>APADNAADARPVDVSVSIFINKIYGVNTLEQTYKVDGYIVAQWTGKPRKTPGDKPLIVENTQIERWINNGLWVPALEFINVVGSPDTGNKRLMLFPDGRVIYNARFLGSFSNDMDFRLFPFDRQQFVLELEPFSYNNQQLRFSDIQVYTENIDNEEIDEWWIRGKASTHISDIRYDHLSSVQPNQNEFSRITVRIDAVRNPSYYLWSFILPLGLIIAASWSVFWLESFSERLQTSFTLMLTVVAYAFYTSNILGRLPYTTYIDQMIIAGYGSIFAAILLIIFAHHRQANGVEDDLLIQRSRLAFPLGFLAIGCVLVIRFFTL[5x]

Pentameric ligand-gated ion channels (pLGICs) mediate synaptic transmission and are sensitive to their lipid environment. We demonstrate that the model pLGIC, ELIC (Erwinia ligand-gated ion channel), is positively modulated by the anionic phospholipid, phosphatidylglycerol, from the outer leaflet of the membrane. To investigate the mechanism of positive modulation by POPG, we determined structures of WT ELIC by single particle cryo-electron microscopy (cryo-EM) in the absence and presence of agonist in MSP1E3D1 nanodiscs with 2:1:1 POPC:POPE:POPG (hereafter referred to as 2:1:1) or POPC. In combination with streamlined alchemical free energy perturbation calculations and functional measurements in asymmetric liposomes, the data support a mechanism by which an anionic phospholipid stabilizes the activated, open-channel state of a pLGIC by specific, state-dependent binding to this site.

Seeking a mutant that remains open in the presence of agonist, we added the mutations P254G (previously shown to slow deactivation) and C300S (previously shown to slow desensitization in the presence of agonist), and produced P254G/C300S/V261Y/G319F/I320F (ELIC5). Strikingly, ELIC5 showed a deactivation rate ~1000× slower than WT and no evidence of desensitization in the presence of 10 mM cysteamine, indicative of profound stabilization of the activated, open-channel state. Consistent with its gain-of-function phenotype, a structure of ELIC5 in 2:1:1 nanodiscs with 10 mM cysteamine, determined at 3.4 Å resolution, yielded an apparent open pore with a pronounced outer leaflet phospholipid-shaped density. Finally, in ELIC5, 9′ rotates away from the pore into an intersubunit space and 16′ opens further, such that the narrowest diameter of the pore is at 2′ (Q233). Two rotameric states of Q233 could be modeled in the structure yielding a minimum pore diameter of 5.6 Å (rotamer 1, ELIC5 CA 1) and 7.3 Å (rotamer 2, ELIC5 CA 2). ELIC5 has the same single channel conductance as WT; this along with its high open probability strongly suggests that the ELIC5 structure represents a functionally-relevant open-channel conformation. The ELIC5 CA structure shows a strong phospholipid density at an outer leaflet site within an intersubunit groove formed by M4, M3 and M1. The β6-β7 loop progressively translates outward from WT apo to WT CA to ELIC5 CA, placing the basic residue, R117, less than 4 Å from the phospholipid headgroup in the ELIC5 CA structure. The outward translation of these structures is linked to a global outward blooming of 4–5 Å of all four transmembrane helices leading to opening of the pore. In the TMD, the outward blooming of the TM helices in the ELIC5 CA structure extends to the bottom of the transmembrane helices, and is associated with an outward translation of 4.7 Å and straightening of M4 below P305, a conserved proline that produces a kink in the M4 helix in non-conducting structures of ELIC.2-chloranyl-~{N}-[(7~{S})-2-methyl-7-phenyl-10-(1~{H}-1,2,3,4-tetrazol-5-yl)-8,9-dihydro-6~{H}-pyrido[1,2-a]indol-7-yl]-4-(1,2,4-triazol-4-yl)benzamide 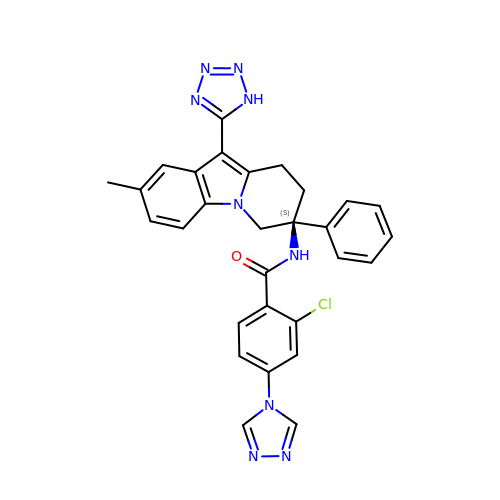| C29 H24 Cl N9 O | TUCDMISJVGVBLL-GDLZYMKVSA-N> GPLGSLKFESDFDFEKANEKFQEVLVDNLEKLNIEDKAEPEVEEKKDAAFYDKK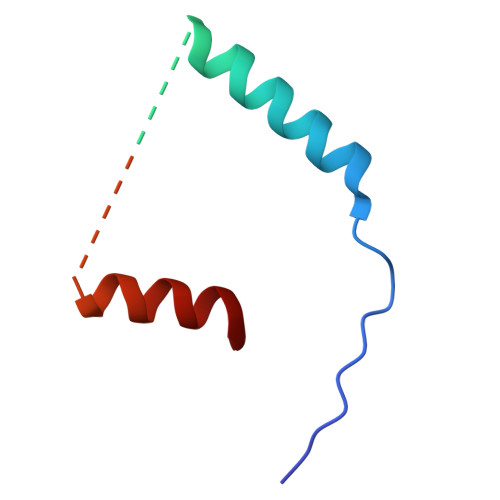TSFFDNISCESLEKAEGKTGRPDWKKERETNQETFG>MIYIIGSGIAGLSAGVALRRAGKKVTLISKRIDGGSTPIAKGGVAASVGSDDSPELHAQDTIRVGDGLCDVKTVNYVTSEAKNVIETFESWGFEFEEDLRLEGGHTKRRVLHRTDETGREIFNFLLKLAREEGIPIIEDRLVEIRVKDGKVTGFVTEKRGLVEDVDKLVLATGGYSYLYEYSSTQSTNIGDGMAIAFKAGTILADMEFVQFHPTVTSLDGEVFLLTETLRGEGAQIINENGERFLFNYDKRGELAPRDILSRAIYIEMLKGHKVFIDLSKIEDFERKFPVVAKYLARHGHNYKVKIPIFPAAHFVDGGIRVNIRG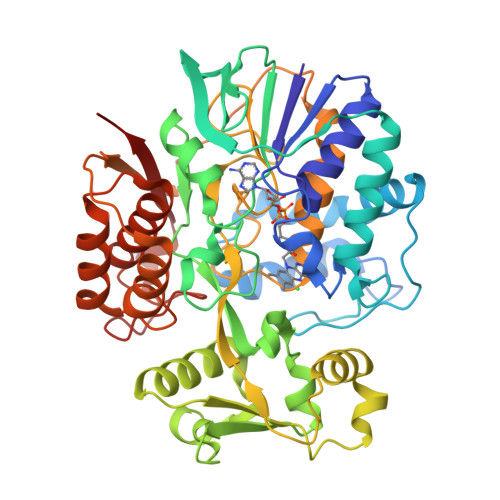ESNIVNLYAIGEVSDSGLHGANRLASNSLLEGLVFGINLPRYVDSSWEGISTDDGIVHSVRISGNKTLSLKEIRRINWENVGIIRNEEKLVKAINTYSSSTQNEAIISYLTALAAEIRKESRGNHFREDYPYKDPNWEKRIYFKLVV[2x]>[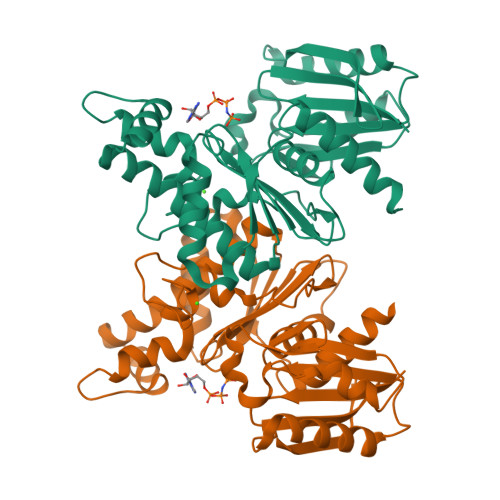2x]MRCLALDIGGTKIASAIVTDGKIEQRQQIATPQADAANAMHDTLANILALYAGQFDYVAVASTGIINHGVLTALNPKNLGGLAEFPLKESIARHTDKPIGLLNDVQAAACAEYKDEDKNAVQNFVFITVSTGVGGGIILERRLLTEPNGVAGHIGHTLADPNGPVCGCGRVGCVEAVAAGRAIEAVSSQWNPPCTPKQAFELFRKNDEKATALIQRSASAIANLIADLVIGLDVQKVVVGGSVGLAEGYLPLVKQYLNTMPHFYHCTVEQARHGQDAGLLGAAWWVADCLKQG>GSHMGGVEVLEVRTGPDAITQIEAYLNPRMGNNIPSEDLYGYSNSINTAFSKASDTPNKDTLPCYSVAVIKLPLLNEDMTCDTILMWEAVSVKTEVVGISSLVNLHQGGKYIYGSSSGCVPVQGTTYHMFAVGGEPLELQGLVASSTATYPDDVVAIKNMKPGNQGLDPKAKALLDKDGKYPVEVWCPDPSKNENTRYYGSFTGGATTPPVMQFTNSVTTVLLDENGVGPLCKGDKLFLSCADIAGVHTNYSETQVWRGLPRYFNVTLRKRIVKNPYP[10x]

Attachment of the LPyV major capsid protein VP1 to receptors on host cells is clearly critical for the restricted tropism of the virus. LPyV VP1 forms a ring-shaped homopentamer in which the five monomers are arranged around a central five-fold axis and connected by extensive interaction surfaces. Sialic acid is a crucial component of the LPyV receptor as removal or modification of cellular sialic acids abolished or modulated LPyV cell binding and infection, but the identity of the sialylated LPyV receptor and its role in tropism are not known. Glycan array and structural analyses show that LPyV VP1 specifically recognizes linear trisaccharides terminating in α2,3-linked sialic acid.

Each LPyV VP1 pentamer contains five oligosaccharide binding sites, which are located at the top of the pentamer, corresponding to the outer surface of the virion. Only some of these binding sites were occupied with ligand, whereas access to the remaining binding sites was blocked by crystal contacts. Both compounds bound in essentially the same manner to each binding site. The terminal Neu5Ac residue, which is best defined by electron density and has low temperature factors (B-factors), inserts deeply into a cleft and engages the protein with multiple contacts. In contrast to most viral sialic acid-binding sites, the LPyV site is not a shallow depression on the protein surface, but a deep cleft that contacts both faces of the Neu5Ac ring, mostly via van der Waals interactions. Consequently, 80% of the accessible surface area of Neu5Ac (317 Å2 of a total of 399 Å2) is buried upon binding. Whereas Neu5Ac in the context of 3SL was readily bound, the analogous α2,6-linked oligosaccharide 6SL was not recognized in both glycan array and crystal soaking experiments. Due to the α2,6-linkage, the overall shape of the trisaccharide is somewhat kinked and differs from the linear orientation found in α2,3-linked compounds. An α2,6-linkage would likely lead to loss of the hydrogen bonds involving Gal and clashes with the BC2cw- or HI-loops of LPyV VP1. The trisaccharide 3SL corresponds to the glycan portion of the ganglioside GM3, a possible receptor candidate. However, the Glc residue in GM3 would most likely be buried in the head group layer of the membrane, and modelling suggests that membrane-bound GM3 would clash with LPyV residue F73 when the Neu5Ac is inserted into the binding pocket.> MSSHTPKLDSCGAEPIHIPGAIQEHGALLVLSAREFSVVQASDNLANYIGVDLPIGAVATEANLPFISVLSAWYSGAASNFRYAWAEKKLDVSAHRSGTLVILEVEKAGVGESAEKLM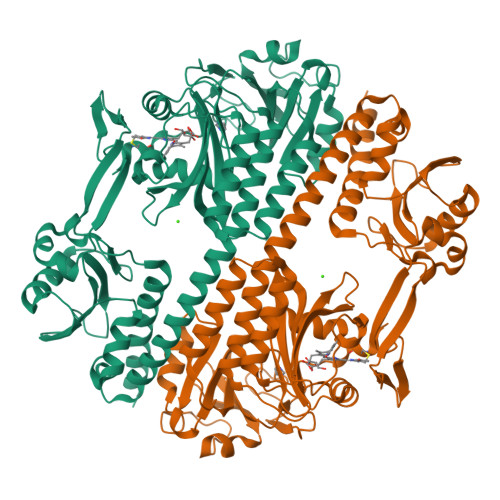GELTSLAKYLNSAPSLEDALFRTAQLVSSISGHDRTLIYDFGLDWSGHVVAEAGSGALPSYLGLRFPAGDIPPQARQLYTINRLRMIPDVDYKPVPIRPEVNAETGAVLDMSFSQLRSVSPVHLEYMRNMGTAASMSVSIVVNGALWGLIACHHATPHSVSLAVREACDFAAQLLSMRIAMEQSSQDASRRVELGHIQARLLKGMAAAAAWVDGLLGGEGEREDLLKQVGADGAALVLGDDYELVGNTPSREQVEELILWLGEREIADVFATDNLAGNYPTAAAYASVASGIIAMRVSELHGSWLIWFRPEVIKTVRWGGDPHKTVQESGRIHPRKSFEIWKEQLRNTSFPWSEPELAAARELRGAIIGIVLRKTEELEHHHHHH> GAMEDENILRNAVNLQVLKFHYPEIESIIDIASHVAVYQFDVGSQKWLKTSIEGTFFLVKDQRARVGYVILNRNSPENLYLFINHPSNVHLVDRYLIHRTENQHVVGLWMFDPND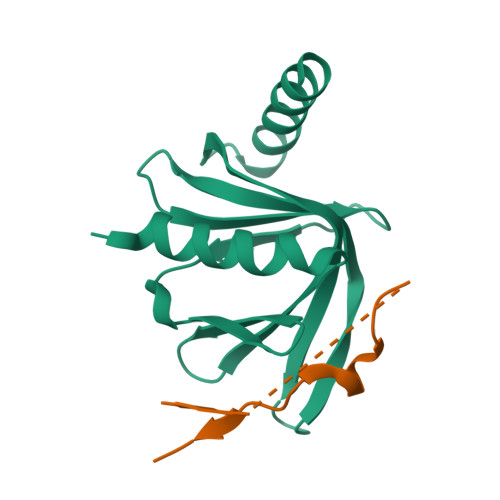MSRIFNIVKESLLR;> GAMSFSSNSSSDTNSILYAGPTFTHSPAASNLPIPTFLHSP>TDKIYDALEKLAEIQKEIAEFLRELIEAAE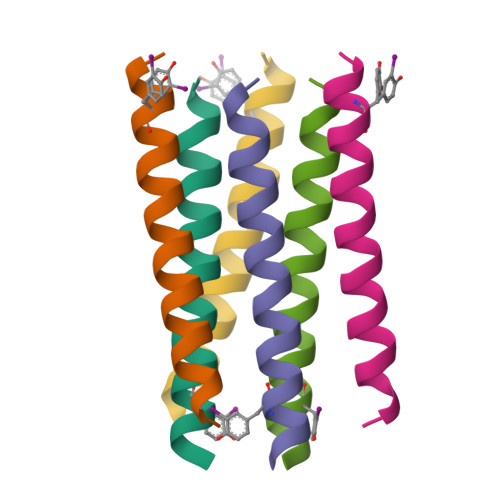KT[2x]> MGSDKIHHHHHHMKTRADLFAFFDAHGVDHKTLDHPPVF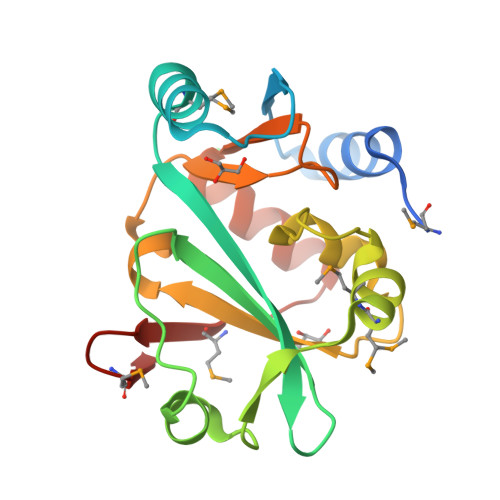RVEEGLEIKAAMPGGHTKNLFLKDAKGQLWLISALGETTIDLKKLHHVIGSGRLSFGPQEMMLETLGVTPGSVTAFGLINDTEKRVRFVLDKALADSDPVNFHPLKNDATTAVSQAGLRRFLAALGVEPMIVDFAAMEVVG> GAMGTTDDVDPEAEYAAWKLRELRRLRRERDAIEARERELAELERRRNLTEEERRAEDEAHLAKQKAE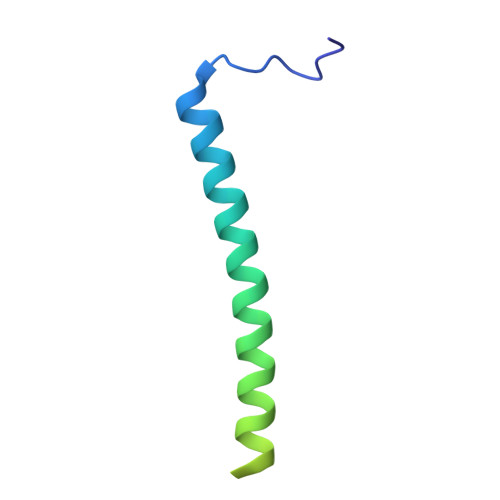KESRGKMGYLQKYFHR>MEEPEEPADSGQSLVPVYIYSPEYVSMCDSLAKIPKRASMVHSLIEAYALHKQMRIVKPKVASMEEMATFHTDAYLQHLQKVSQEGDDDHPDSIEYGLGYDCPATEGIFDYAAAIGGATITAAQCLIDGMCKVAINWSGGWHHAKKDEASGFCYLNDAVLGILRLRRKFERILYVDLDLHHGDGVEDAFSFTSKVMTVSLHKFSPGFFPGTGDVSDVGLGKGRYYSVNVPIQDGIQDEKYYQNCESVLKEVYQAFNPKAVVLQLGADTIAGDPMCSFNMTPVGIGKCLKYILQWQLATLILGGGGYNLANTARCWTYLTGVILGKTLSSEIPDHEFFTAYGPDYVLEITPSCRPDRNEPHRIQQILNYIKGNLKHVVIE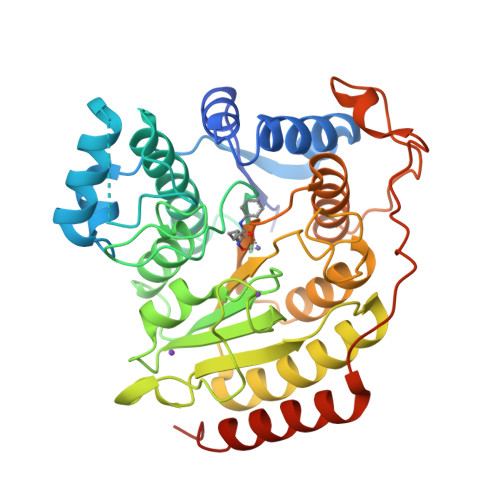GRGSHHHHHH[2x]>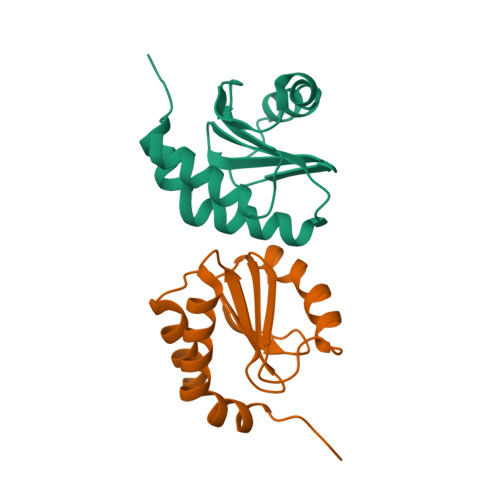[4x]GPIIENCAAFIEKTMSKYAITLSDGTILKSTIKNETLKKTFPILKNLLKDQIPTGSSFFKLPVVFFRVTDNVIVILLTNEKENIILSMFELFSTQFAEKLALEYPRTYE3-[2-azanyl-5-[2-(phenoxymethyl)-1,3-thiazol-4-yl]phenyl]propanoic acid | C19 H18 N2 O3 S | 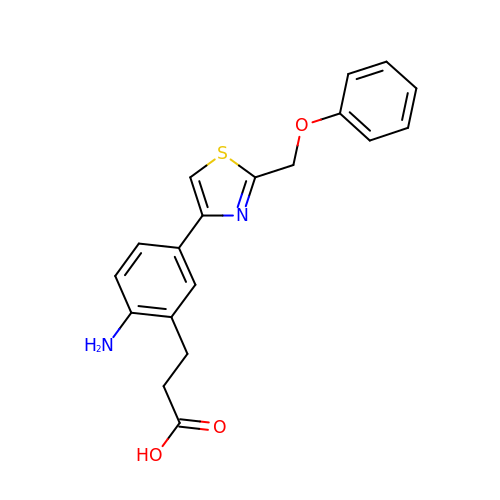RXPAQUQGUPYCSG-UHFFFAOYSA-N> MPVPNPTMPVKGAGTTLWVYKGSGDPYANPLSDVDWSRLAK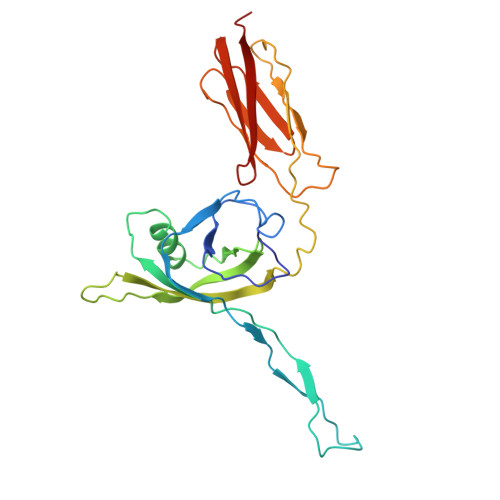VKDLTPGELTAESYDDSYLDDEDADWTATGQGQKSAGDTSFTLAWMPGEQGQQALLAWFNEGDTRAYKIRFPNGTVDVFRGWVSSIGKAVTAKEVITRTVKVTNVGRPSMAEDRSTVTAATGMTVTPASTSVVKGQSTTLTVAFQPEGVTDKSFRAVSADKTKATVSVSGMTITVNGVAAGKVNIPVVSGNGEFAAVAEITVTAS> MKIYVDGREVIINDNERNLLEALKNVGIEIPNLCYLSEASIYGACRMCLVEINGQITTSCTLKPYEGMKVKTNTPEIYEMRRNILELILATHNRDCTTCDRNGSCKLQKYAEDFGIRKIRFEALKKEHVRDESAPVVRDTSKCILCGDCVRVCEEIQGVGVIEFAKRGFESVVTTAFDTPLIETECVLCGQCVAYCPTGALSIRNDIDKLIEALESDKIVIGMIAPAVRAAIQEEFGIDEDVAMAEKLVSFLKTIGFDKVFDVSFGADLVAYEEAHEFYERLKKGERLPQFTSCCPAWVKHAEHTYPQYLQNLSSVKSPQQALGTVIKKIYARKLGVPEEKIFLVSFMPCTAKKFEAEREEHEGIVDIVLTTRELAQLIKMSRIDINRVEPQPFDRPYGVSSQAGLGFGKAGGVFSCVLSVLNEEIGIEKVDVKSPEDG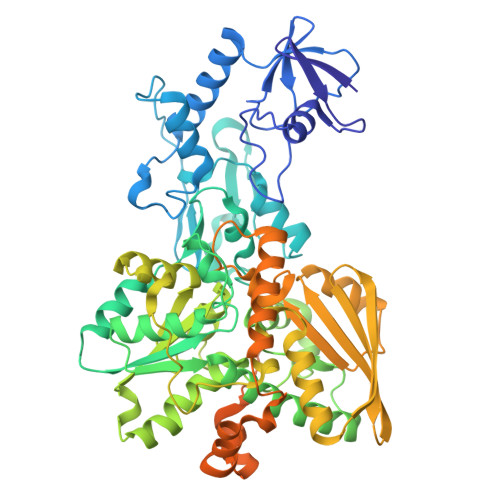IRVAEVTLKDGTSFKGAVIYGLGKVKKFLEERKDVEIIEVMACNYGCVGGGGQPYPNDSRIREHRAKVLRDTMGIKSLLTPVENLFLMKLYEEDLKDEHTRHEILHTTYRPRRRYPEKDVEILPVPNGEKRTVKVCLGTSCYTKGSYEILKKLVDYVKENDMEGKIEVLGTFCVENCGASPNVIVDDKIIGGATFEKVLEELSKNG>[3x]AAPTAYTPLDVAQAY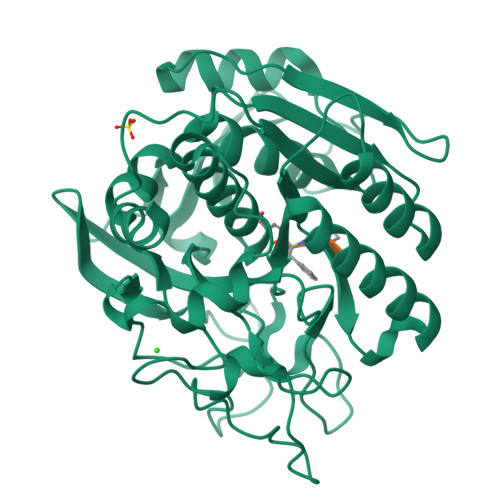QFPEGLDGQGQCIAIIELGGGYDEASLAQYFASLGVPAPQVVSVSVDGASNQPTGDPSGPDGEVELDIEVAGALAPGAKFAVYFAPNTDAGFLDAITTAIHDPTLKPSVVSISWGGPEDSWTSAAIAAMNRAFLDAAALGVTVLAAAGDSGSTDGEQDGLYHVDFPAASPYVLACGGTRLVASGGRIAQETVWNDGPDGGATGGGVSRIFPLPAWQEHANVPPSANPGASSGRGVPDLAGNADPATGYEVVIDGEATVIGGTSAVAPLFAALVARINQKLGKAVGYLNPTLYQLPADVFHDITEGNNDIANRAQIYQAGPGWDPCTGLGSPIGVRLLQALLPSASQPQP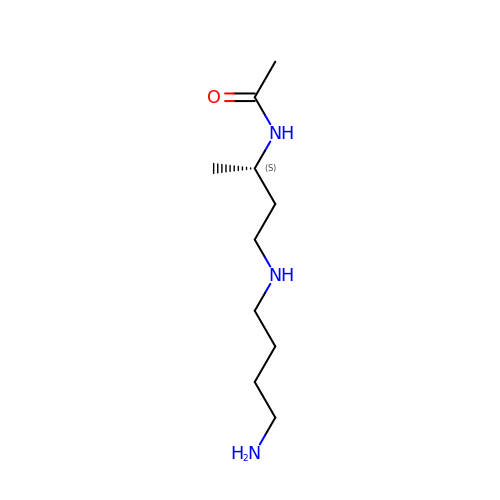N-{(1S)-3-[(4-aminobutyl)amino]-1-methylpropyl}acetamide | C10 H23 N3 O | NCHUZACAGJBRLA-VIFPVBQESA-N>[2x]MSETTQTSQSLYQALWNSADVLRSKMDANDYKSYLLGMVFYKYLSDKMLFFVAETMEEETESLDEALAVYRKYYEDEETHEDLLAVITDEMSYAIHPDLTFTALVERVNDGSFQLEDLAQGFRDIEQSDELYENLFEDIDLYSKKLGATPQKQNQTVAAVMKELAVLDVAGHAGDMLGDAYEYLIGQFATDSGKKAGEFYTPQPVAKLMTQIAFLGREDKQGFTLYDATMGSGSLLLNAKRYSRQPQTVVYFGQELNTSTYNLARMNMILHGVPIENQFLHNADTLDEDWPTQEPTNFDGVLMNPPYSA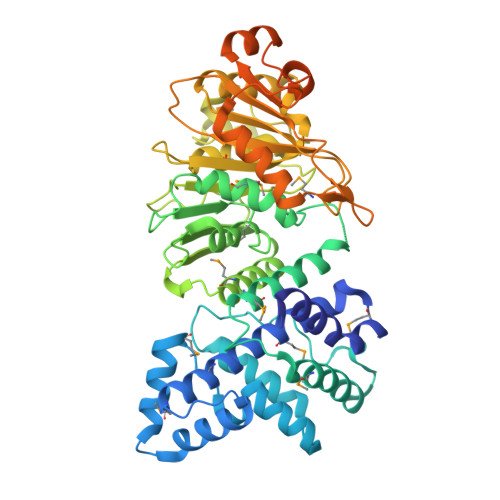KWSASSGFMDDPRFSPFGKLAPKSKADFAFLLHGYYHLKQDNGVMAIVLPHGVLFRGNAEGTIRKALLEEGAIDTVIGLPANIFFNTSIPTTVIILKKNRTNRDVYFIDASKEFDKGKNQNIMTDAHIEKILNAYKSREDIDKFAHLASFEEIVENDYNLNIPRYVDTFEEEEVEPLTEIVAKINQTNATIESQTASLLDMLGQLHGTTPEADEELKAFVKAFKGLEHHHHHH>MINHKIFPTADAVVKSLADDMLAYSQQGQPVHISLSGGSTPKMLFKLLASQPYANDIQWKNLHFWWGDERCVAPDDAESNYGEANALLFSKINMPAQNIHRILGENEPQAEAERFAQAMAHVIPTENGTPVFDWILLGVGADGHTASLFPGQTDYADANLSVVASHPESGQ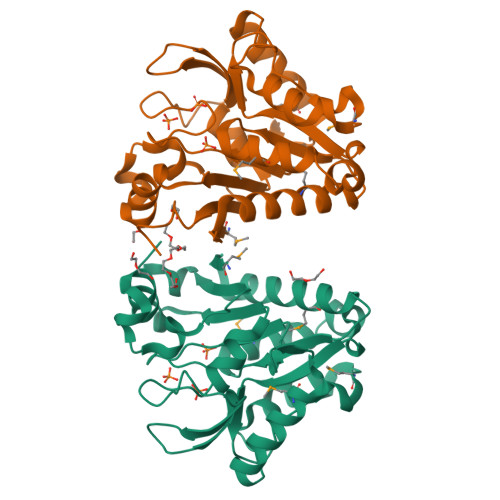LRVSKTAKVLQAAKRISYLVLGAGKAEIVEQIHTTPAEQLPYPAAKIHSTSGVTEWYLDSDAAAKIA[2x]>MPQAFFSHNNKDKKIVLEVLEHLRQSLVATWIDQQSIPGGGSLIQQIIAGISKSQYFLAFLSNEYLKSDWCWDELEQAYALHQKGKVKIIPILLTNRAQLDLNALTDARRNFLESILTRLKYVEFDPHNMTRSLGSVAEALWQNEAVRFEPIRMIKVNGTELQVVEFKIPGSNLPVDFLHHWDLKIEDFIATSPNEQKPVKFDVPVALYGPGPNWLYAFLTLPFKNRNTVFVFNSRTSEYICVYSKSAGLAPGMVLKGHHHHH[22x]

Here we investigated a protein containing a CARF domain fused Toll/interleukin-1 receptor (TIR) domain, Cat1. We found that Cat1 provides immunity by cleaving and depleting NAD+ molecules from the infected host, inducing a growth arrest that prevents viral propagation. Cat1 forms dimers that stack upon each other to generate long filaments that are maintained by bound cOA ligands, with stacked TIR domains forming the NAD+ cleavage catalytic sites. Further, Cat1 filaments assemble into unique trigonal and pentagonal networks that enhance NAD+ degradation.

The cryo-EM structure of cA4-bound Cat1 shows that the complex assembles into filamentous structures, forming intricate higher-order networks. The fundamental repeat unit of this topology is defined by the two-fold symmetric alignment of a pair of TIR-CARF monomers, involving central positioning of the CARF domains and outwards positioning of the TIR domains. Successive stacking of TIR-CARF dimers, anchored in place by bound cA4 positioned between them, results in formation of linear filaments, exhibiting a slight twist, as part of the higher-order filament network. While analyzing the higher-order filament network of cA4-Cat1 complex, we noticed that the dimeric repeat units associate with two adjacent Cat1 dimers forming a surprising trigonal assembly. The inter-repeat unit association is mediated by amino acid backbone interactions between a small loop formed by N158 and G159 residues joining the β1- β2 strands of the CARF domain (designated β1β2-loop) of repeat unit 1 and the N103 and A104 residues present at the TIR domain of the adjacent Cat1 dimer. In this trigonal assembly, the third Cat1 dimer does not pair up with the first Cat1 dimer, but instead it tilts around the center of the dimer (see blue arrow implying a shift below the plane). The tilt causes a shift of the TIR domain, one of which points towards the trigonal assembly, below the plane of repeat units 1 and 2 by 24 Å, thereby forming the helical bundle by bringing it close to the CARF domain β1β2-loop of the Cat1 dimeric unit which initiates the next turn. Thus, the trigonal Cat1 dimer assembly gives rise to a spiral filament bundle with a triangular pore in the middle. Three Cat1 dimers are present in each turn of the spiral bundle with an overall diameter of 170 Å and the bundle is closely packed without any pitch (gap between turns). To test the importance of these supra-structures for Cat1 activity, we made deletions of residues N103-A104 and N158 to eliminate the backbone interactions that facilitate high-order assembly.Cd2+-binding aptamers have been extensively utilized in the development of Cd2+-detecting devices; however, the underlying mechanisms remain elusive. This study reports four Cd2+-bound DNA aptamer structures, representing the only Cd2+-specific aptamer structures available to date. In all the structures, the Cd2+-binding loop (CBL-loop) adopts a compact, double-twisted conformation and the Cd2+ ion is mainly coordinated with the G9, C12 and G16 nucleotides. Other nucleotides of the loop and the G8–C18 pair of the stem also affect the Cd2+ binding, via proper folding and/or stabilizing the conformation of the CBL-loop.

To this end, in this study, T10A, T10C and T10G variants of DNA1 were synthesized. Though not as strong as the native DNA1, ITC analysis confirmed that the T10A variant could bind Cd2+; the KD value of T10A was found to be 3.83 ± 0.282 μM. The binding of Cd2+ by the T10A variant could be further supported by the T10A–Cd2+ complex structure. The structure belongs to the C2 space group and contains two T10A–Cd2+ complexes per asymmetric unit. The low RMSD value (0.55 Å) indicates that the overall folding of the two T10A–Cd2+ complexes is very similar. The relative orientations between the stem and the CBL-loop regions are different in the T10A–Cd2+ complex and the native DNA1–Cd2+ structure. However, the conformations of the CBL-loops are very similar; the RMSD value between the CBL-loops of the two structures is ∼0.33 Å. The nucleobase of A10 shows two alternative conformations. Similarly to T10 in the native DNA1–Cd2+ structure, A10 points away from any nucleotide within the CBL-loop. The packing of the T10A–Cd2+ and the native DNA1–Cd2+ complexes is very different in their crystal lattices.

>[2x]GACGACGGGATCACAGTCCGTTGTC2'-DEOXYCOFORMYCIN 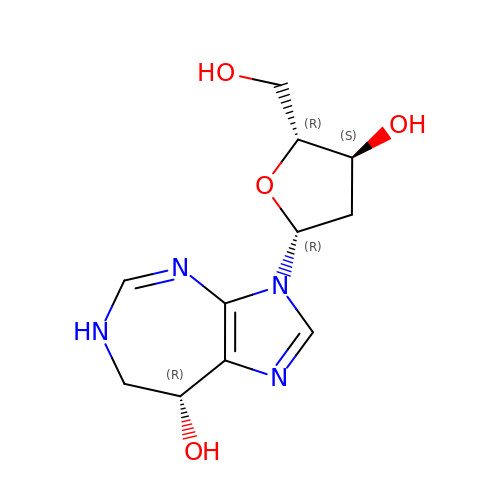| C11 H16 N4 O4 | FPVKHBSQESCIEP-JQCXWYLXSA-N>[4x]KACTRECGNLGFGICPRSEGSPLNPICINCCSGYKGCNYYNSFGKFICEGESDPKRPNACTFNCDPNIAYS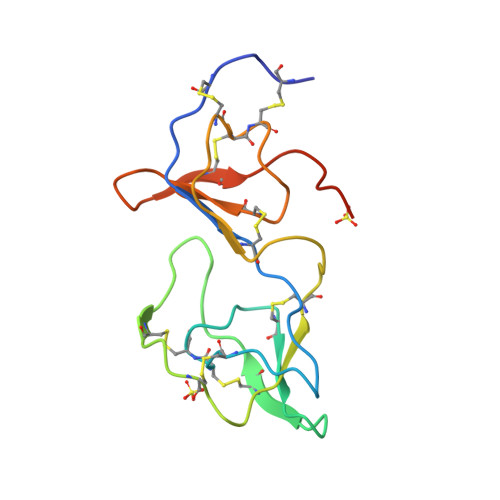RCPRSQGKSLIYPTGCTTCCTGYKGCYYFGKDGKFVCEGESDEPKANMYPVM>GSHMKSSVVGSERKRGMQLEDLKQQLQQAEEALVAKQEVIDKLKEEAEQHKIVMETVPVLKAQADIYKADFQA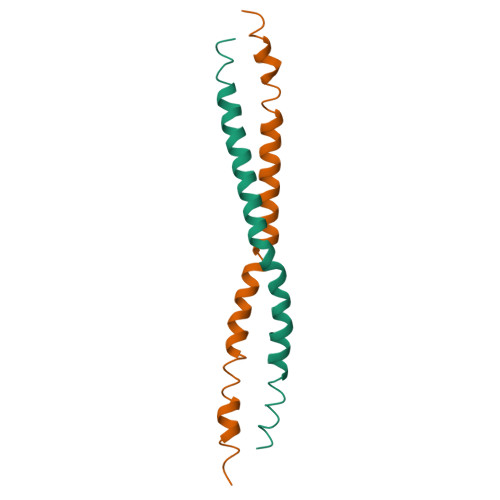ERQAREKLAEKKELLQEQLEQLQ[2x]> MFKAQATFSRYSAAVSLLLLFSGAAQAAPQSITTLPLQPDGENRWRLPAGEYQGQFTIEQPMQLRCEPGAVIQSQGQGSSLLISAPDVLVEGCTLYEWGSDLTAMDSAVFILPAAERAQISNNRMRGPGFGVFVDGTRDVQVIGNEIDGDAGVRSQDRGNGIHLFAVSGARVLHNHVRNARDGIYIDTSNGNHLEGNVIEDVRYGVHYMFANENSLIDNVTRRTRTGYALMQSRKLTVTGNRSEQDQNYGILMNYITYSTITGNFVSDVQRGDTGGDSMISGGEGKALFIYNSLFNTIENNHFEKSSLGIHLTAGSEDNRISGNAFVGNQQQVKYVASRTQEWSVDGRGNYWSDYLGWDRNNDGLGDIAYEPNDNVDRLLWLYPQVRLLMNSPSIEVLRWVQRAFPVIKSPGVQDSHPLMKLPTEKLLTEKQEPTS;>MNAVEIQGVSQRYGSMTVLHDLNLNLGEGEVLGLFGHNGAGKTTSMKLILGLLSPSEGQVKVLGRAPNDPQVRRQLGYLPENVTFYPQLSGRETLRHFARLKGAALTQVDELLEQVGLAHAADRRVKTYSKGMRQRLGLAQALL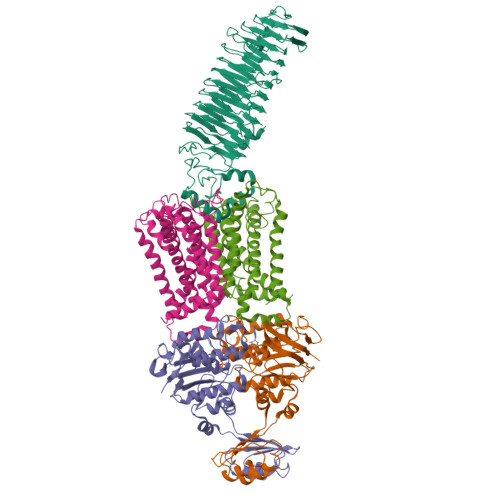GEPRLLLLDQPTVGLDPIATQDLYLLIDRLRQRGTSIILCSHVLPGVEAHINRAAILAKGCLQAVGSLSQLRAEAGLPVRIRASGISERDSWLQRWTDAGHSARGLSESSIEVVAVNGHKLVLLRQLLGEGEPEDIEIHQPSLEDLYRYYMERAGDVRAQEGRL[2x];>[2x]MNQVWNIARKELSDGLRNRWLLAISLLFAVLAVGIAWLGAAASGQLGFTSIPATIASLASLATFLMPLIALLLAYDAIVGEDEGGTLMLLLTYPLGRGQILLGKFVGHGLILALAVLIGFGCAALAIALLVEGVELGMLFWAFGRFMISSTLLGWVFLAFAYVLSGKVNEKSSAAGLALGVWFLFVLVFDLVLLALLVLSEGKFNPELLPWLLLLNPTDIYRLINLSGFEGSGSAMGVLSLGADLPVPAAVLWLCLLAWIGVSLLLAYAIFRRRLT>[2x]MGSSHHHHHHSSGLVPRGSHMPATHHSSATSAERPTVVGRIPVLDVRPVVQRGRRPAKAVTGESFEVSATVFREGHDAVGANVVLRDPRGRPGPWTPMRELAPGTDRWGATVTAGETGTWSYTVEAWGDPVTTWRHHARIKIPAGLDTDLVLEEGARLYERAAADVPGREDRRELLAAVDALRDESRPAASRLAAALTPQVDAVLARHPLR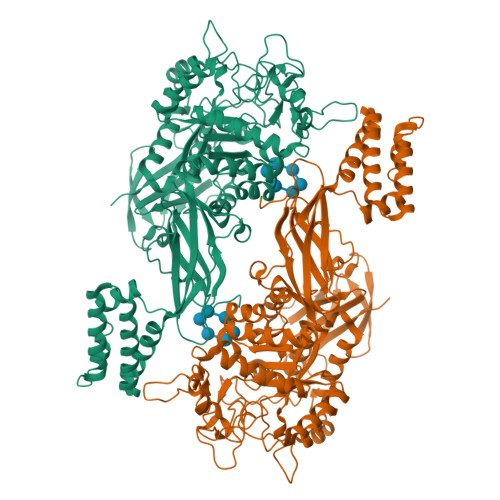DLVTSSDPLPLLVERERALYGAWYEFFPRSEGTPHTPHGTFRTAARRLPAIAAMGFDVVYLPPIHPIGTTHRKGRNNTLSATGDDVGVPWAIGSPEGGHDSIHPALGTLDDFDHFVTEAGKLGLEIALDFALQCSPDHPWVHKHPEWFHHRPDGTIAHAENPPKKYQDIYPIAFDADPDGLATETVRILRHWMDHGVRIFRVDNPHTKPVAFWERVIADINGTDPDVIFLAEAFTRPAMMATLAQIGFQQSYTYFTWRNTKQELTEYLTELSGEAASYMRPNFFANTPDILHAYLQHGGRPAFEVRAVLAATLSPTWGIYSGYELCENTPLREGSEEYLDSEKYQLKPRDWTRAAREGTTIAPLVTRLNTIRRENPALRQLRDLHFHPTDKEEVIAYSKRQGSNTVLVVVNLDPRHTQEATVSLDMPQLGLDWHESVPVRDELTGETYHWGRANYVRLEPGRTPAHVCTVLRPSHPQIGGSHTT> MENIAVVGIANLFPGSQAPDQFWQQLLEQQDCRSKATAVQMGVDPAKYTANKGDTDKFYCVHGGYISDFNFDASGYQLDNDYLAGLDDLNQWGLYVTKQALTDAGYWGSTALENCGVILGNLSFPTKSSNQLFMPLYHQVVDNALKAVLHPDFQLTHYTAPKKTHADNALVAGYPAALIAQAAGLGGSHFALDAACASSCYSVKLACDYLHT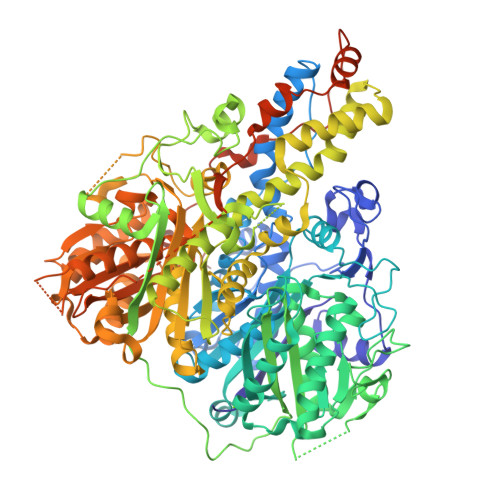GKANMMLAGAVSAADPMFVNMGFSIFQAYPANNVHAPFDQNSQGLFAGEGAGMMVLKRQSDAVRDGDHIYAIIKGGALSNDGKGEFVLSPNTKGQVLVYERAYADADVDPSTVDYIECHATGTPKGDNVELRSMETFFSRVNNKPLLGSVKSNLGHLLTAAGMPGMTKAMLALGKGLIPATINLKQPLQSKNGYFTGEQMPTTTVSWPTTPGAKADKPRTAGVSVFGFGGSNAHLVLQQPTQTLETNFSVAKPREPLAIIGMDSHFGSASNLAQFKTLLNNNQNTFRELPEQRWKGMESNANVMQSLQLRKAPKGSYVEQLDIDFLRFKVPPNEKDCLIPQQLMMMQVADNAAKDGGLVEGRNVAVLVAMGMELELHQYRGRVNLTTQIEDSLLQQGINLTVEQREELTNIAKDGVASAAQLNQYTSFIGNIMASRISALWDFSGPAITVSAEENSVYRCVELAENLFQTSDVEAVIIAAVDLSGSIENITLRQHYGPVNEKGSVSECGPVNESSSVTNNILDQQQWLVGEGAAAIVVKPSSQVTAEQVYARIDAVSFAPGSNAKAITIAADKALTLAGISAADVASVEAHASGFSAENNAEKTALPTLYPSASISSVKANIGHTFNASGMASIIKTALLLDQNTSQDQKSKHIAINGLGRDNSCAHLILSSSAQAHQVAPAPVSGMAKQRPQLVKTIKLGGQLISNAIVNSASSSLHAIKAQFAGKHLNKVNQPVMMDNLKPQGISAHATNEYVVTGAANTQASNIQASHVQASSHAQEIAPNQVQNMQATAALEHHHHHH>MFEKILLSNPSAENPSSLRPRKGIIIGLGQVGLACAYSMLIQDCFDELVLQDIASDKLEGEVMDFSHGMPFIPPTDIKAGTIANEGRN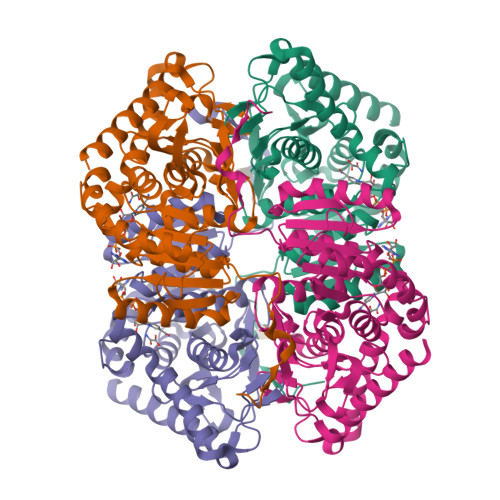ADIVIITAGVAQKEGESRLSLLERNIAIYKKILADVVKYCPEAIILVVTNPVDIMTYATLKITGFPSSRIIGSGTVLDTARFRTLLAKEMDIDPRSVHAYIIGEHGDSEVPVWSTANVGGMKLVPNTWADLPEDEKATLSGIFQKVQNAAYDIIKLKGYTSYAIGLATTDIVKAILNSQERILTVSGLMTGMYGIEDVCLSIPRVVSERGIIKTVNLTLSEDEEKLLQQSAKMLKEVFDKINYHHHHHH[4x]> NSLFNQEVQIP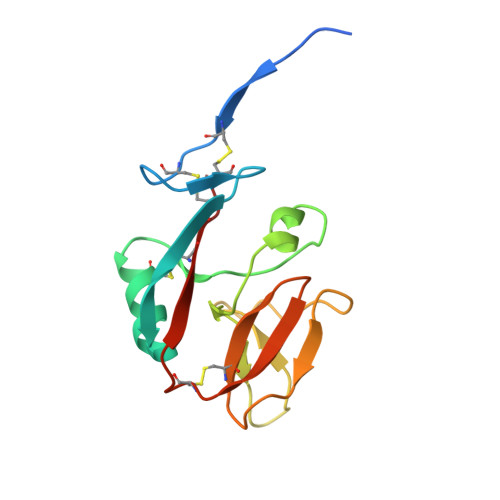LTESYCGPCPKNWICYKNNCYQFFDESKNWYESQASCMSQNASLLKVYSKEDQDLLKLVKSYHWMGLVHIPTNGSWQWEDGSILSPNLLTIIEMQKGDCALYASSFKGYIENCSTPNTYICMQRTV> AADSTGYDKDLVEALERDIISQNPNVRWDDIADLVEAKKLLKEAVVLPMWMPEFFKGIRRPWKGVLMVGPPGTGKTLLAKAVATECKTTFFNVSSSTLTSKYRGESEKLVRLLFEMARFYSPATIFIDEIDSICSRRGTSEEHEASRRVKAELLVQMDGVG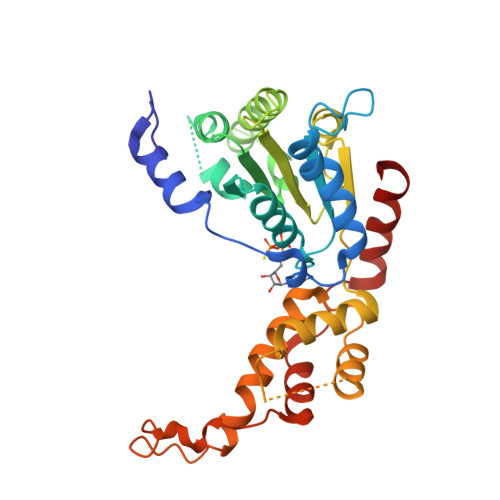GTSENDDPSKMVMVLAATNFPWDIDEALRRRLEKRIYIPLPSAKGREELLRISLRELELADDVDLASIAENMEGYSGADITNVCRDASLMAMRRRIEGLTPEEIRNLSKEEMHMPTTMEDFEMALKKVSKSVSAADIERYEKWIFEFG>[4x]MIASVRGEVLEVALDHVVIEAAGVGYRVNATPATLATLRQGTEARLITAMIVREDSMTLYGFPDGETRDLFLTLLSVSGVGPRLAMAALAVHDAPALRQVL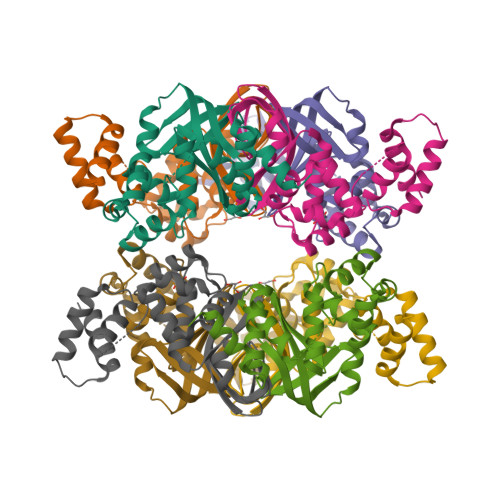ADGNVAALTRVPGIGKRGAERMVLELRDKVGVAATGGALSTNGHAVRSPVVEALVGLGFAAKQAEEATDTVLAANHDATTSSALRSALSLLGKAR Bemnifosbuvir (AT-527) and AT-752 are guanosine analogues currently in clinical trials against several RNA viruses. Here, we show that these drugs require a minimal set of 5 cellular enzymes for activation to their common 5′-triphosphate AT-9010, with an obligate order of reactions. Crystal structures of human histidine triad nucleotide binding protein 1, adenosine deaminase-like protein 1, guanylate kinase 1, and nucleoside diphosphate kinase at 2.09, 2.44, 1.76, and 1.9 Å resolution, respectively, with cognate precursors of AT-9010 illuminate the activation pathway from the orally available bemnifosbuvir to AT-9010, pointing to key drug–protein contacts along the activation pathway.

ADALP1 is a deaminase acting on N6-substituted purine nucleoside monophosphates. ADALP1 is thus able to accept the 2′-C-methyl, 2′-F modifications on the ribose part, as well as several substituents on the N6-position. The solved ADALP1 structure adopts an α/β-barrel architecture similar to that of ADAs, with the essential Zn2+ ion tightly bound in the vicinity of the catalytic center. The asymmetric unit contains 8 copies of the protein. Although ADALP1 was co-crystallized with the substrate AT-8003, the product AT-8001 was found bound at the active site. The compound is found in all 8 chains, and all the chains found in the asymmetric unit closely superimpose (RMSD of approximately 0.26 Å) except for the minor loop and N- and C-terminal ends. The structural zinc is coordinated by side chains of 4 residues (His 24, His 26, His 208, and Asp 293) and a water molecule, in a trigonal bipyramidal geometry. AT-8001 is buried in a closed hydrophobic pocket that can only accommodate a monophosphate compound checked and stabilized by Asn 28, His 74, Ser 106, and Thr 107. Once the substrate is bound, the catalytic water attacks the purine C6, which likely stays at this location while the methylamine is leaving in the opposite exit channel. In the case of ADALP1, unlike HINT1, the substrate and products are superimposable in the crystal structure, indicating that this complex should be reliable and useful for drug design.

>[8x]MIEAEEQQPCKTDFYSELPKVELHAHLNGSISSHTMKKLIAQKPDLKIHDQMTVIDKGKKRTLEECFQMFQTIHQLTSSPEDILMVTKDVIKEFADDGVKYLELRSTPRRENATGMTKKTYVESILEGIKQSKQENLDIDVRYLIAVDRRGGPLVAKETVKLAEEFFLSTEGTVLGLDLSGDPTVGQAKDFLEPLLEAKKAGLKLALHLSEIPNQKKETQILLDLLPDRIGHGTFLNSGEGGSLDLVDFVRQHRIPLELCLTSNVKSQTVPSYDQHHFGFWYSIAHPSVICTDDKGVFATHLSQEYQLAAETFNLTQSQVWDLSYESINYIFASDSTRSELRKKWNHLKPRVLHI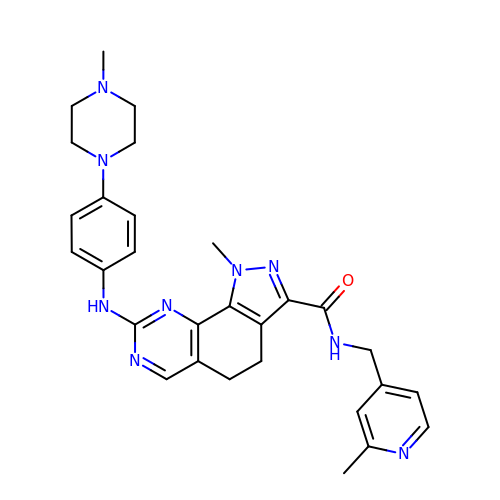1-METHYL-8-{[4-(4-METHYLPIPERAZIN-1-YL)PHENYL]AMINO}-N-[(2-METHYLPYRIDIN-4-YL)METHYL]-4,5-DIHYDRO-1H-PYRAZOLO[4,3-H]QUINAZOLINE-3-CARBOXAMIDE | C29 H33 N9 O | BMPXFYMECYEYOL-UHFFFAOYSA-N> MKVAVLPGDGIGPEVTEAALKVLRALDEAEGLGLAYEVFPFGGAAIDAFGEPFPEPTRKGVEEAEAVLLGSVGGPKWDGLP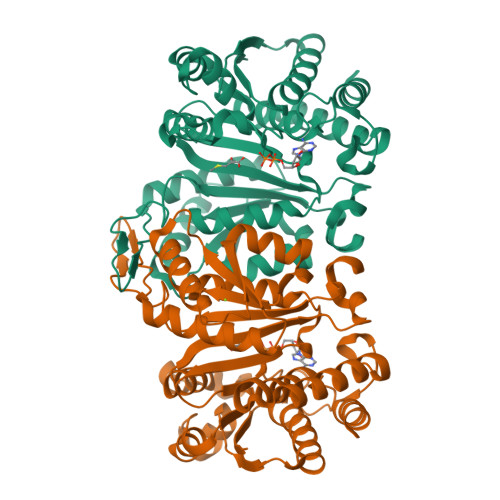RKIRPETGLLSLRKSQDLFANLRPAKVFPGLERLSPLKEEIARGVDVLIVRELTGGIYFGEPRGMSEAEAWNTERYSKPEVERVARVAFEAARKRRKHVVSVDKANVLEVGEFWRKTVEEVGRGYPDVALEHQYVDAMAMHLVRSPARFDVVVTGNIFGDILSDLASVLPGSLGLLPSASLGRGTPVFEPVHGSAPDIAGKGIANPTAAILSAAMMLEHAFGLVELARKVEDAVAKALLETPPPDLGGSAGTEAFTATVLRHLA> MGSSHHHHHHSQDQTSTATFREDFHSLRAGGLNWDSLPLRLFGKGNAKFWDPADIDFTRDAEDWQGLTEEERRSVAMLCSQFIAGEEAVTQDLQPFMAAMAAEGRFGDEMYLTQFCFEEAKHTQVFRLWMDAVGLTGDLHSHVAENPGYRAIFYEELPRSLNALHDDPSPANQVRASVTYNHVVEGTLALTGYFAWQKICRSRGILPGMQEVVRRIGDDERRHMAWGTFTCRRHVAADESNWDVVQEQMQHLLPLAVTQIQWRPEDAPEETPFRLDIDELAAYASDRAGR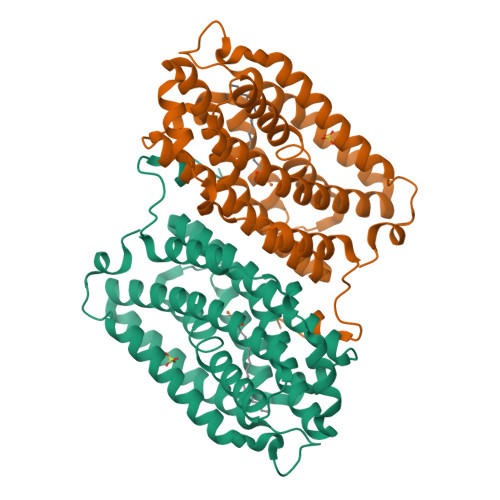RLGAISAARGVPVEQIDVDASPEQLEDQFGVEDAAALEKA>MSTLANLTEVLFRLDFDPDTAVYHYRGQTLSRLQCRTYILSQASQLARLLKPGDRVVLALNDSPSLACLFLACIAVGAIPAVINPKSREQALADIAADCQASLVVREADAPSLSGPLAPLTLRAAAGRPLLDDFSLDALVGPADLDWSAFHRQDPAAACFLQYTSGSTGAPKGVMHSLRNTLGFCRAFATELLALQAGDRLYSIPKMFFGYGMGNSLFFPWFSGASALLDDTWPSPERVLENLVAFRPRVLFGVPAIYASLRPQ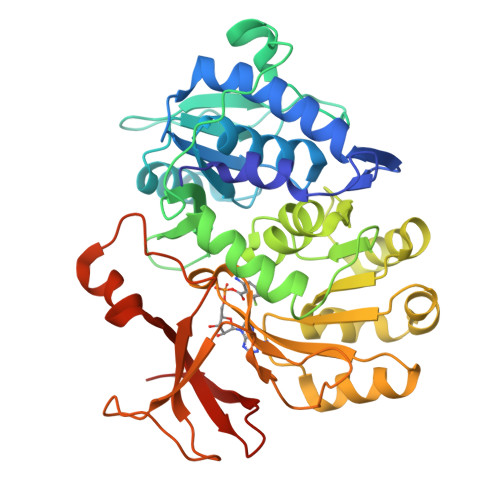ARELLSSVRLAFSAGSPLPRGEFEFWAAHGLEICDGIGATEVGHVFLANRPGQARADSTGLPLPGYECRLVDREGHTIEEAGRQGVLLVRGPGLSPGYWRASEEQQARFAGGWYRTGDLFERDESGAYRHCGREDLEHHHHHH[4x]> GMAEAKSRVGRPSGDTQNRDKLILAARNLFIERPYAQVSIREIASLAGTDPGLIRYYFGSKEKLFSTMIHETAMPVLAQLHKARRETRQESPAALLQTYYSVMSKHPHFPRLMLRIAGLDQSLPENAEVTKAFYEVVNFENIAIFQRLKDKNLLKDDVDAHCAQLSFFAMMVFPFIVPENLLERVGIELTPDFLQL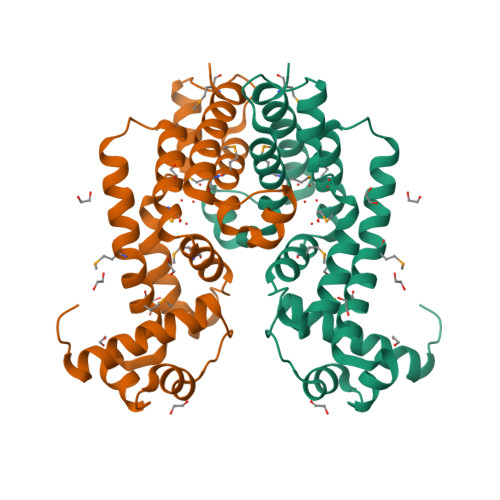LAEQNTRLLQRGLMDVKDERDE> MQFRSIIRIVGLLLALFSVTMLAPALVALLYRDGAGVPFVTTFFVLLFCGAMCWFPNRRHKHELKSRDGFLIVVLFWTVLGSAGSLPFLI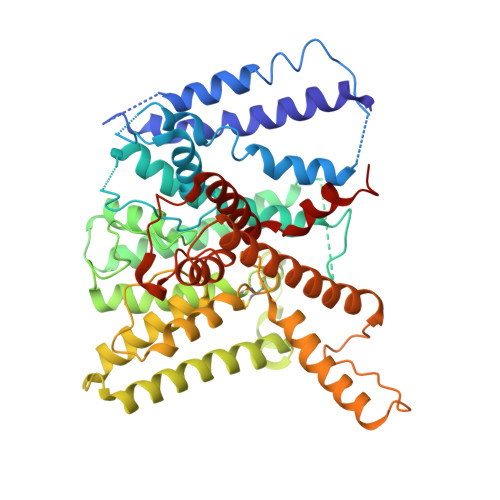ADNPNISVTDAFFESFSALTTTGATVIVGLDELPKAILFYRQFLQWFGGMGIIVLAVAILPVLGIGGMQLYRAEIPGPVKDTKMTPRIAETAKALWYIYLSLTIACAVAFWLAGMTPFDAISHSFSTIAIGGFSTHDASMGYFDSYAINLITVVFLLISACNFTLHFAAFASGGVHPKYYWKDPEFRAFIFIQVLLFLVCFLLLLKHHSYTSPYDAFDQALFQTVSISTTAGFTTTGFADWPLFLPVLLLFSSFIGGCAGSTGGGMKVIRILLLTLQGARELKRLVHPRAVYTIKVGGSALPQRVVDAVWGFFSAYALVFVVCMLGLIATGMDELSAFSAVAATLNNLGPGLGEVALHFGDVNDKAKWVLIVSMLFGRLEIFTLLILLTPTFWRS>MENYLIDNLDRGILEALMGNARTAYAELAKQFGVSPETIH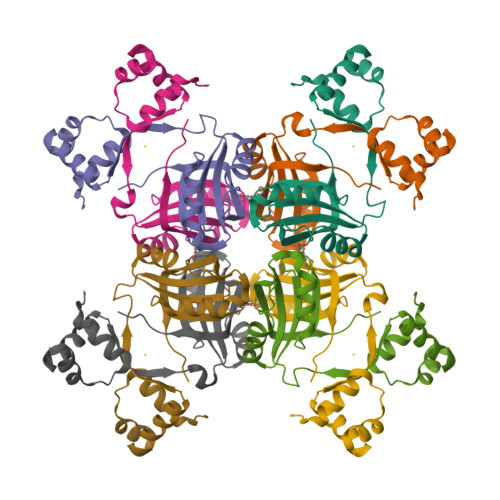VRVEKMKQAGIITGARIDVSPKQLGYDVGCFIGIILKSAKDYPSALAKLESLDEVTEAYYTTGHYSIFIKVMCRSIDALQHVLINKIQTIDEIQSTETLIVLQNPIMRTIKP[2x]> HGYVTFPIARQR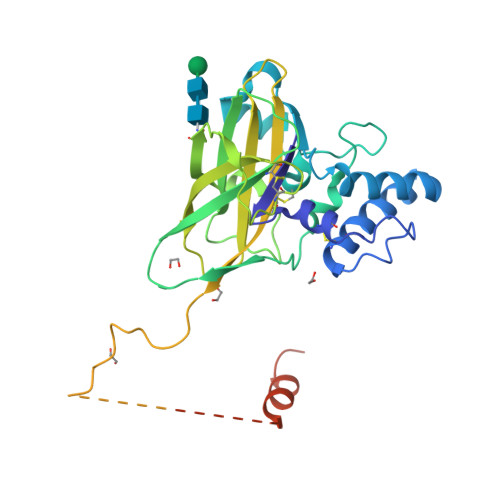RCNVQGGFWWPPEGTNIPDPMCRAAYQYVFNKVLSEGGSTSQAASAAQYMFQQDNEYAALAGPNFRDICWIKEQVVPDYLCAAGADTWRIRPFGDKTGMDIVGSWPPTVIPLENNFVNTIPIELEFCPTAIHEPSYFEVYVTTPEFNVYRDKVTWPLLELVFNSTVPLVNRRADSLCTANARVYRMIVPVPYRQTQFVIYVRWQRIDPVGEGFYNCVDAVFANRPGPDPEDMIPPPPAEEDCDYTDSQGNRYCPFSTFSNSYYSNREHYNHKHDYNRYSNYYDHNTYTYNYGKYNKNKYSDTTYNNRAWEIAYAGYTEDHTGLNRQTECDGISRFCVSTVRNRVY>GSKNLIGRHLRLGSVEEQPFMFFATEGCEGNDCWSGMVNDMVVKLSEDLGFTYEYIQPDDRKFGALNKTTNEWNGMIRDLLDDKT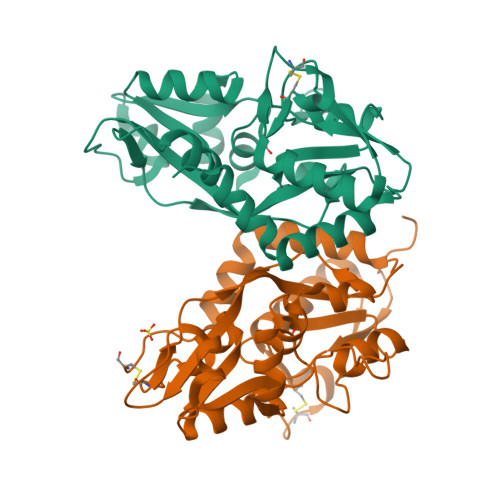DMIAIDLSTNSARKSAIDYSFPFMDAGIKAVVKGEGTTLNQVLELLDQDKYKWGVIGSRHPETLLKTHRDSRYSRLVDEGVELKDLNHAIETLRGGLFVFIDEGPVLAHNLISDCDVFSVGEEFQSFEYAFGLPKDSPYKSLIDSHLLKFREEGFIDILWEKWSSGNSVCS[2x]> MPVSVMRLTNINKGIIKLLPQIVTLIILITAIPQLAKLTWRVVFPVSPEDISAL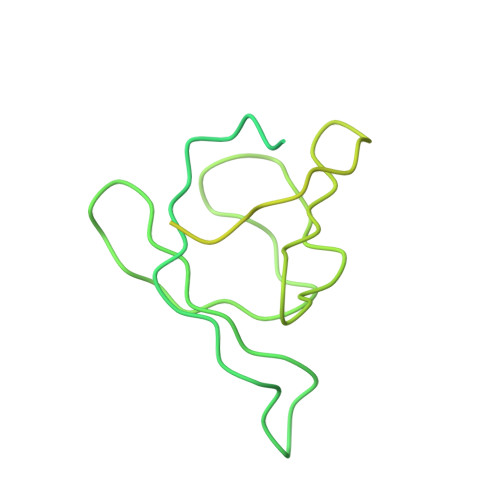PLTMPPAADPELKNVRPAFTLFGLAVKNSPTPTDAASLNQVPVSSLKLRLAGLLASSNPARSIAIIEKGNQQVSLSTGDPLPGYDARIAAILPDRIIVNYQGRKEAILLFNDSRAPSPPPTAAGNPPLVKRLREQPQNILTYLSISPVLSGDKLLGYRLNPGKDASLFRQSGLQANDLAIALNGIDLRDQEQAQQALQNLADMTEITLTVEREGQRHDIAFALGDE>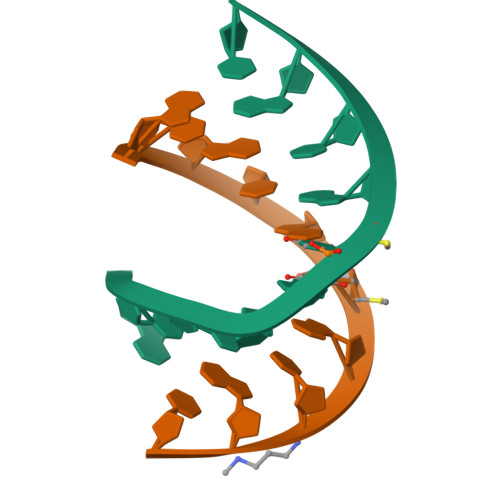[2x]GCGTAUACGC> MTQMLTRPDVDLVNGMFYADGGAREAYRWMRANEPVFRDRNGLAAATTYQAVLDAERNPELFSSTGGIRPDQPGMPYMIDMDDPQHLLRRKLVNAGFTRKRVMDKVDSIGRLCDTLIDAVCERGECDFVRDIAAPLPMAVIGDMLGVLPTERDMLLKWSDDLVCGLSSHVDEAAIQKLMDTFAAYTEFTKDVITKRRAEPTDDLFSVLVNSEVEGQRMSDDEIVFETLLILIGGDETTRHTLSGGTEQLLRHRDQWDALVADVDLLPGAIEEMLRWTSPVKNMCRTLTADTVFHGTELRAGEKIMLMFESANFDESVFGDPDNFRIDRNPNSHVAFGFGTHFCLGNQLARLELRLMTERVLR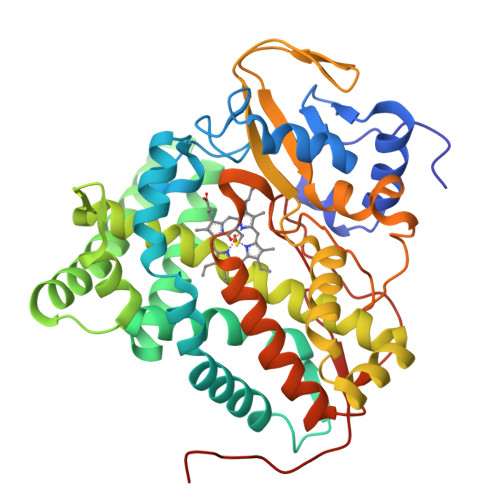RLPDLRLADDAPVPLRPANFVSGPESMPVVFTPSAPVLAHHHHHH> MSAVEISPDVLVYKSPLTEQSTEYASISNNSDQTIAFKVKTTAPKFY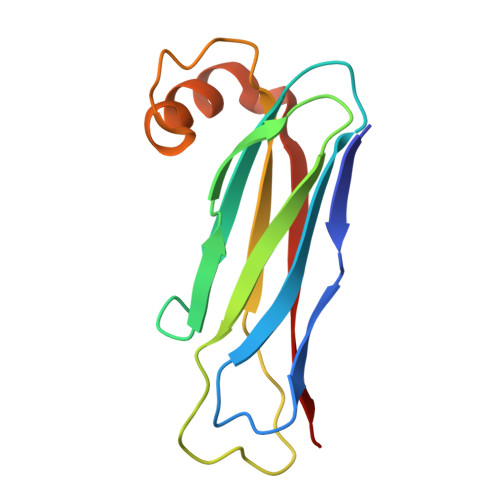CVRPNAAVVAPGETIQVQVIFLGLTEEPAADFKCRDKFMVITLPSPYDLNGKAVADVWSDLEAEFKQQAISKKIKVKYLIS> GPKVEQAVETEPEPELRQQTEWQSGQRWELALGRFWDYLRWVQTLSEQVQEELLSSQVTQELRALMDETMKELKAYKSELEEQLTPVAEETRARLSKELQAAQARLGADMEDVVGRLVQYRGEVQAMLGQST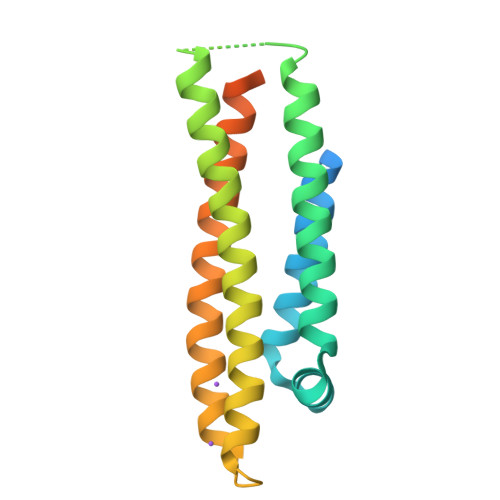EELRVRLASHLRKLRKRLLRDADDLQKRLAVYQAGAREGAERGLSAIRERLGPLVEQGRVR>NLKMEIILTLSQGLKKYYGKILRLLQLTLEEDTEGLLEWCKRNLGLDCDDTFFQKRIEEFFITGEGHFNEVLQFRTPGTLSTTESTPAGLPTAEPFKSYFAKGFLSIDSGYYSAKCYSGTSN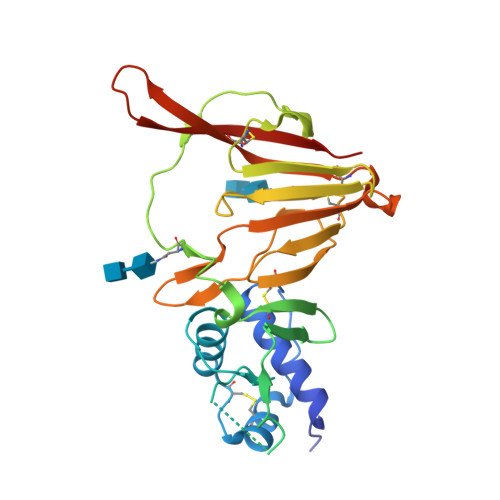SGLQLINITRHSTRIVDTPGPKITNLKTINCINLKASIFKEHREVEINVLLPQVAVNLSNCHVVIKSHVCDYSLDIDGAVRLPHIYHEGVFIPGTYKIVIDKKNKLNDRCTLFTDCVIKGREVRKGQSVLRQYKTEIRIGKASTGS[2x]>MSTTDQGETGKACPYPFAEMERLEIHPEYNRLRDAGELGRVLMPYGGETWLATSWEDVAKVFVDPRFSRSATLGKDVPRVLPAIQDQPVIMLMDPPEHTRLRRLATKALTSRRMEALRPRTQEVADDLIDKMLAKGAPADLMEDFALPLPIIMICELLGVPIEDQTKFRTWSDQMLSNGAYSQEVVMAAGQSLYLYLSELIAERRKQDTNDLLGSLVRARDKDDRLSETELVGFAVTLLIAGYETTANAIGNSVYTLLTHPEKLAELRKDLSLIPKAVDELLRIIPIAKQAS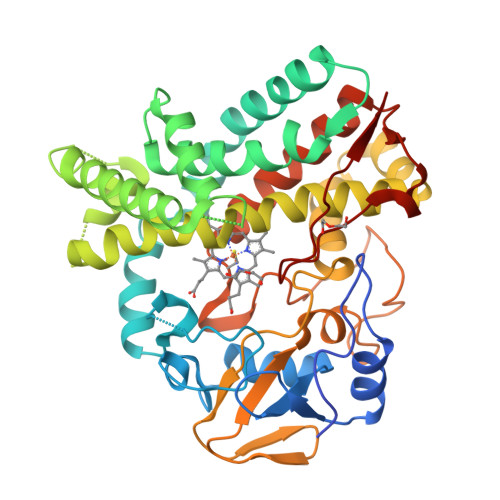WVRMAVEDVELSGTIVKAGEAVAIQTHSANTDPKVYDHPEEIDFHRTSNPHMSLGHGAHHCMGAQLVRVEMQTALGSLISRIPALRFAVPEPRIKFLRGRLVPSLEALPLTW[2x]> MADYKDDDDKGTDYKDDDDKLEVLFQGPMSLRIDVDTNFPECVVDAGKVTLGTQQRQEMDPRLREKQNEIILRAVCALLNSGGGIIKAEIENKGYNYERHGVGLDVPPIFRSHLDKMQKENHFLIFVKSWNTEAGVPLATLCSNLYHRERTSTDVMDSQEALAFLKCRTQTPTNINVSNSLGPQAAQGSVQYEGNINVSAAALFDRKRLQYLEKLNLPESTHVEFVMFSTDVSHCVKDRLPKCVSAFANTEGGYVFFGVHDETCQVIGCEKEKIDLTSLRASIDGCIKKLPVHHFCTQRPEIKYVLNFLEVHDKGALRGYVCAIKVEKFCCAVFAKVPSSWQVKDNRVRQLPTREWTAWMMEADPDLSRCPEMVLQLSLSSATPRSKPVCIHKNSE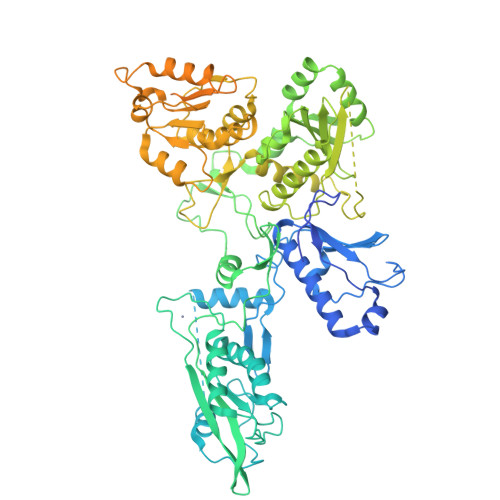CLKEQQKRYFPVFSDRVVYTPESLYKELFSQHKGLRDLINTEMRPFSQGILIFSQSWAVDLGLQEKQGVICDALLISQNNTPILYTIFSKWDAGCKGYSMIVAYSLKQKLVNKGGYTGRLCITPLVCVLNSDRKAQSVYSSYLQIYPESYNFMTPQHMEALLQSLVIVLLGFKSFLSEELGSEVLNLLTNKQYELLSKNLRKTRELFVHGLPGSGKTILALRIMEKIRNVFHCEPANILYICENQPLKKLVSFSKKNICQPVTRKTFMKNNFEHIQHIIIDDAQNFRTEDGDWYGKAKFITQTARDGPGVLWIFLDYFQTYHLSCSGLPPPSDQYPREEINRVVRNAGPIANYLQQVMQEARQNPPPNLPPGSLVMLYEPKWAQGVPGNLEIIEDLNLEEILIYVANKCRFLLRNGYSPKDIAVLFTKASEVEKYKDRLLTAMRKRKLSQLHEESDLLLQIGDASDVLTDHIVLDSVCRFSGLERNIVFGINPGVAPPAGAYNLLLCLASRAKRHLYILKASV>NAKRIEGLDSNVWVEFTKLAADPSVVNLGQGFPDISPPSYVKEELSKAAFIDNMNQYTRGFGHPALVKALSCLYGKIYQRQIDPNEEILVAVGAYGSLFNSIQGLVDPGDEVIIMVPFYDCYEPMVRMAGAVPVFIPLRSKPTDGMKWTSSDWTFDPRELESKFSSKTKAIILNTPHNPLGKVYTRQELQVIADLCVKHDTLCISDEVYEWLVYTGHTHVKIATLPGMWERTITIGSAGKTFSVTGWKLGWSIGPAHLIKHLQTVQQNSFYTCATP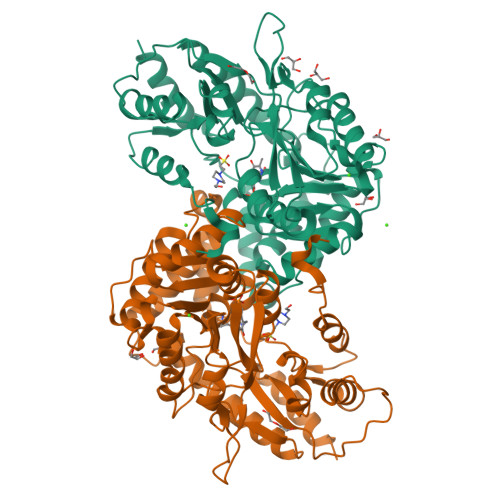LQAALAEAFWIDIKRMDDPECYFNSLPKELEVKRDRMVRLLNSVGLKPIVPDGGYFIIADVSSLGADLSDMNSDEPYDYKFVKWMTKHKKLTAIPVSAFCDSKSKPHFEKLVRFCFIKKDSTLDAAEEIFRAWN[2x]One protein family common to humans, C. parvum and in fact all eukaryotes is the group of tyrosine 3-monooxygenase/tryptophan 5-monooxygenase activation proteins (YWHA), also known as 14-3-3 proteins. All 14-3-3 proteins are dimers, with each subunit comprised of nine α-helices framing a peptide-binding cleft. The dimer is shaped like the letter “W” from one angle, with an un-partitioned bicameral pocket where a substrate protein is held at two typically phosphorylated sites in the two component clefts. The parasite Cryptosporidium parvum has three 14-3-3 proteins: Cp14ε, Cp14a and Cp14b, with only Cp14ε similar to human 14-3-3 proteins in sequence, peptide-binding properties and structure.

While Cp14ε conformably binds a number of known 14-3-3 ligands and Cp14a attracts none, the third C. parvum 14-3-3 protein in our study stands out by interacting with a peptide that is a phosphorylated copy of the last six amino acids in its own C-terminus: LLT(pS)AFF – a motif hitherto not known to be relevant in the context of 14-3-3 proteins. Protomer 1 follows the standard 14-3-3 architecture, albeit with the helix αB1 atypically disordered (and hence not visible in the crystallographic structure). The bound tail features a phosphorylated serine and the sequence LLT(pS)AFF. This serine, which was found to be phosphorylated in the crystal structure despite the fact that the protein was expressed in E. coli, interacts with the Arg79-Arg153-Arg154 triad just as the mode 1 peptide does in Cp14ε, with the backbone of Cp14b's tail tightly aligned with the peptide RAI(pS)LP and fitting in the binding groove in a very similar way. In contrast, the other subunit of Cp14b, namely protomer 2, has a disordered C-terminus in our crystallographic structure; however, this polypeptide displays its own unique feature. Specifically, the helices αA2 and αB2 appear as one continuous helix, behaving like a bent spring given room to relax and straighten. The resulting “super” helix, dubbed αAB2, is shifted from where αA and αB are typically found. In its new position, αAB2 blocks access to the binding groove and potentially contributes to inhibition of Cp14b's ability to bind another protein, as seen in Figs. 5D and 5E from two different angles. With protomer 2 adopting a conformation with only 8 helices, Cp14b can no longer form a dimer in the same way as other 14-3-3 proteins, which rely on helices A and B configured as a bent spring. The novel dimer, held together by hydrophobic interaction, does not form a merged and undivided substrate cradle. Instead, the two binding grooves face opposite directions and are separated by helices αC1, αD1, αAB2, αC2 and αD2. The division and twisting of this cavity makes it impossible for the chaperone to hold a substrate in the standard way and potentially forms a third mode of inhibition for Cp14b.

>[4x]MGSSHHHHHHSSGRENLYFQGITEKNMKLSEGAYRAKLADMVGNYKDVIKVLTESSDFRDNSLILLLAGSLRNRVTSIRNSLKSIKSQEEKLRKEKSLNNEFIQVIEDIKRDFEESILLESEDVIRIIDDNLLMYSEEGARAFCIKLKGDLMRYKAEILKDEEKNQCIKQAVEFYEDALQRERSFLEKYPSDPLYLATILNYTILKYDLLGNPEGAMKFANRAIQAAENSRSDSEQFSENTEKLLKILRDNVSQWEQGCSGLLTSAFF>[4x]SNAMTSLSSRPGLRRASFLQRGAWRWLREAPPAAAFAARGLLGSGRIDDDRLAAAADEVLDAFPLLRVNFVDDDGLWMRTRENADALVRSDLRGHPDPQARCVELLRADRDRPTDPERDPLVRLHLVRLSET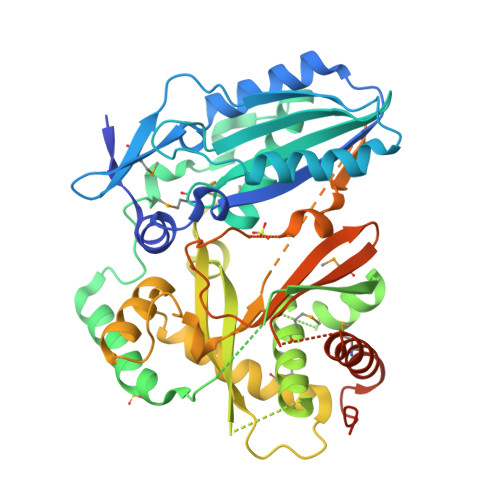DVVLGVVAHQMLLDARSRYMVLGAVWQAYYGRFRPAQYRDFAEVADFHPLDRETVRVARHRWWSRRLPALPVRGGDGGPVGPPETSRLRVPGSRWQALTEPGGPLGGNGSLAMAALTAWWLWTQGAGTGTDTGAGTGTGKDSLYLSTEVDLRDHLQLGSVVGPLTDRVVFGVDLTGLREPSFRDLMSRTQAGFLDAVVHYLPYHDVVDLAVDLGVVTPPRVAARWDVAVHLCRNAPSSSLTRGERTLAELGVSIELFREADLIGGDTRSATDTWDGTDTWDGTTTDLSVGELGEDMVIVLDQRRTHPAGGGSALLDGLDAAMAQAVADPSAPLPHSTVDTTTQSTVDKDTVDRNTAHENEE Phage satellite P4 polarity suppression protein, Psu, a building block of the viral capsid, inhibits hexameric transcription termination factor, ρ, by presently unknown mechanisms. The ρ hexamer adopts an NTPase-inactive, washer-like, open-ring conformation until NTPs (preferentially ATP) are engaged and RNA is bound at the SBS, leading to ring closure and RNA entrapment inside the ring. Our cryogenic electron microscopy structures of ρ-Psu complexes show that Psu dimers clamp two inactive, open ρ rings and promote their expansion to higher-oligomeric states. ATPase, nucleotide binding and nucleic acid binding studies revealed that Psu hinders ρ ring closure and traps nucleotides in their binding pockets on ρ.

A ρ variant harboring a P167L substitution has been observed to bind Psu more tightly than wt ρ38,43. Consistently, we observed a more pronounced shift in the SEC elution volume for ρP167L-Psu mixtures, even in the absence of nucleotides, as compared to wt ρ. We, therefore, also determined cryoEM structures of ρP167L-ATPγS-Psu complexes. The results showed that ρP167L associates with Psu in a similar manner as wt ρ, with a preference for the complex II constellation. In complex II, two hexameric ρ rings are bridged by five Psu dimers that connect ρ(A) subunit 6 with ρ(B) subunit 2, ρ(A) subunit 5 with ρ(B) subunit 3, etc. ATP or ATPγS are bound similarly between all neighboring ρ CTDs in the ρ-ATP/ATPγS-Psu or ρP167L-ATPγS-Psu assemblies. The ρP167L-Psu complex exhibited a ~seven-fold higher mant-ATPγS affinity compared to ρP167L alone (Kd = 2.1 µM). The mant-ATPγS association and dissociation rates of the complex were more than five-fold and ~40-fold lower, respectively, compared to ρP167L alone. The drastic decrease of the mant-ATPγS dissociation rate in the presence of Psu suggests that, once nucleotide is bound, Psu effectively hinders its release.

>[12x]MNLTELKNTPVSELITLGENMGLENLARMRKQDIIFAILKQHAKSGEDIFGDGVLEILQDGFGFLRSADSSYLAGPDDIYVSPSQIRRFNLRTGDTISGKIRPPKEGERYFALLKVNEVNFDKPENARNKILFENLTPLHANSRLRMERGNGSTEDLTARVLDLASLIGRGQRGLIVAPPKAGKTMLLQNIAQSIAYNHPDCVLMVLLIDERPEEVTEMQRLVKGEVVASTFDEPASRHVQVAEMVIEKAKRLVEHKKDVIILLDSITRLARAYNTVVPASGKVLTGGVDANALHRPKRFFGAARNVEEGGSLTIIATALIDTGSKMDEVIYEEFKGTGNMELHLSRKIAEKRVFPAIDYNRSGTRKEELLTTQEELQKMWILRKIIHPMGEIDAMEFLINKLAMTKTNDDFFEMMKRS;>MESTALQQAFDTCQNNKAAWLQRKNELAAAEQEYLRLLSGEGRNVSRLDELRNIIEVRKWQVNQAAGRYIRSHEAVQHISIRDRLNDFMQQHGTALAAALAPELMGYSELTAIARNCAIQRATDALREALLSWLAKGEKINYSAQDSDILTTIGFRPDVASVDDSREKFTPAQNMIFSRKSAQLASRQSV[10x]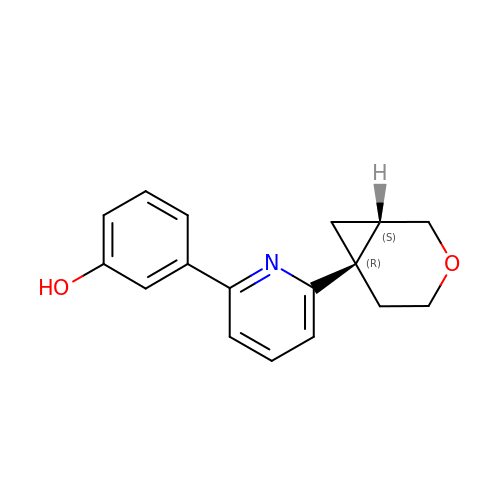3-[6-[(1~{S},6~{R})-3-oxabicyclo[4.1.0]heptan-6-yl]pyridin-2-yl]phenol | C17 H17 N O2 | LKFXAVVNPRARMY-DYVFJYSZSA-N> AVGPFNSVAEAA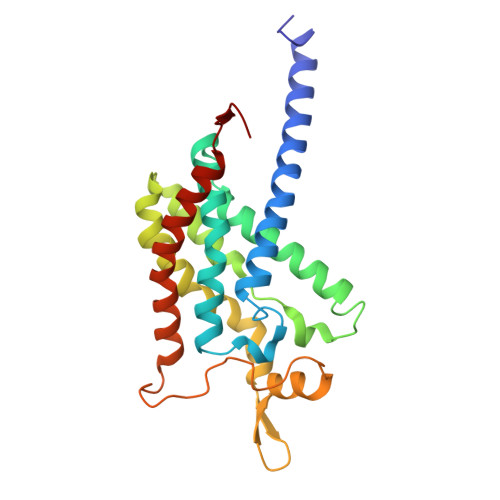GCVQTVDWMLLVLLFFAVLGGYHVHFMLTAGDWDFWVDWKDRRMWPTVVPILGVTFCAASQAFWWVNFRLPFGAVFAALGLLIGEWINRYVNFWGWTYFPISLVFPSALIVPAIWLDVILLLSGSYVITAVVGSLGWGLLFYPNNWPAIAAFHQATEQHGQLMTLADLIGFHFVRTSMPEYIRMVERGTLRTFGKDVVPVAAFFSGFVSMMVYFLWWFMGRWYSTTKVIDTI Here, we visualize, for the model phage T5, how host recognition and SE can be achieved via the interaction of different phage proteins with the same receptor in the Escherichia coli outer membrane. The receptor for phage T5 was identified as the outer membrane (OM) TonB-dependent transporter (TBDT) FhuA almost 50 y ago. To elucidate the mechanism of SE via potential TBDT structure modulation, we report here the cryo-EM structure of the FhuA–pb5 complex and the X-ray crystal structure of the FhuA–Llp complex. Our structures show that the phage lipoprotein Llp exploits the known allostery in the plug of FhuA in the opposite direction as during ferrichrome import (i.e., from the periplasmic side to the extracellular side).

We succeeded in solving the FhuA–pb5 structure via cryo-EM, using complex purified in decylmaltopyranoside at ∼3.1 Å resolution. The FhuA–Pb5 structure shows that pb5 is an elongated molecule with one end inserted into the extracellular lumen of the FhuA barrel and with its long axis approximately perpendicular to the OM plane. Pb5 inserts four loops (numbered L1 to L4 from the N terminus) into the extracellular lumen of FhuA. With the exception of EL1-EL3, all FhuA loops contact pb5, resulting in a large interface area of ∼2140 Å2 as analyzed via PISA. Pb5 completely fills the extracellular lumen of FhuA and occludes the ferrichrome binding site, explaining why addition of purified pb5 to E. coli inhibits growth under iron-starved conditions. Interestingly, pb5 binding does not cause conformational changes in the TonB box, and the structure of the plug in FhuA–pb5 is identical to that in apo FhuA, despite the fact that ferrichrome and pb5 both contact Phe115 and Tyr116 of the plug. The LPS molecule that is present in FhuA X-ray crystal structures is clearly visible in the cryo-EM map. Interestingly, the region at the other end of pb5 that most likely interacts with pb4 is poorly ordered but present in the cryo-EM density and only visible at low contours. Combined with data placing pb5 at the very tip of the central tail fiber, and the loss of tail tips when detergent-purified FhuA is incubated with T5 (13), we propose that the disorder observed in the pb4-interacting part of pb5 is caused by FhuA binding and leads to the dissociation of the tail tip. To our knowledge, our structural data for FhuA–pb5 provide the most direct evidence to date for the view that DNA transfer does not occur via the FhuA channel, as originally proposed based on single-channel electrophysiology.

> AVEPKEDTITVTAAPAPQESAWGPAATIAARQSATGTKTDTPIQKVPQSISVVTAEEMALHQPKSVKEALSYTPGVSVGTRGASNTYDHLIIRGFAAEGQSQNNYLNGLKLQGNFYNDAVIDPYMLERAEIMRGPVSVLYGKSSPGGLLNMVSKRPTTEPLKEVQFKAGTDSLFQTGFDFSDSLDDDGVYSYRLTGLARSANAQQKGSEEQRYAIAPAFTWRPDDKTNFTFLSYFQNEPETGYYGWLPKEGTVEPLPNGKRLPTDFNEGAKNNTYSRNEKMVGYSFDHEFNDTFTVRQNLRFAENKTSQNSVYGYGVCSDPANAYSKQCAALAPADKGHYLARKYVVDDEKLQNFSVDTQLQSKFATGDIDHTLLTGVDFMRMRNDINAWFGYDDSVPLLNLYNPVNTDFDFNAKDPANSGPYRILNKQKQTGVYVQDQAQWDKVLVTLGGRYDWADQESLNRVAGTTDKRDDKQFTWRGGVNYLFDNGVTPYFSYSESFEPSSQVGKDGNIFAPSKGKQYEVGVKYVPEDRPIVVTGAVYNLTKTNNLMADPEGSFFSVEGGEIRARGVEIEAKAALSASVNVVGSYTYTDAEYTTDTTYKGNTPAQVPKHMASLWADYTFFDGPLSGLTLGTGGRYTGSSYGDPANSFKVGSYTVVDALVRYDLARVGMAGSNVALHVNNLFDREYVASCFNTYGCFWGAERQVVATATFRF;> MSFFAGKLNNKSILSLRRGSGGDTNQHINPDSQTIFHSDMSHVIITETHSTGLRLDQGAGDYYWSEMPSRVTQLHNNDPNRVVLTEIEFSDGSRHMLSGMSMGVGAKAYGIINPQIMSQGGLKTQITASADLSLDVGYFNTGTSGTIPQKLRDGTGCQHMFGAFSGRRGFASSAMYLGGAALYKSAWSGSGYVVADAGTLTIPSDYVRHPGARNFGFNAIYVRGRSCNRVLYGMEGPNYTTGGAVQGASSSGALNFTYNPSNPESPKYSVGFARADPTNYAYWESMGDPNDSANGPIGIYSEHLGIYPSKITWYVTNLVYNGSGYNIDGGLFNGNDIKLSPREFIIKGVNVNNTSWKFINFIEKNFNVGNRADFRDVGCNLSKDSPSTGISGIATFGLPTTESNNAPSIKGGNVGGLHANVVSIYNFLPSASWYVSSNPPKIGNNYGDVWSENLLPLRLLGGSGSTILSGNIVFQGNGSVHVGTVGLDLNSSRNGAIVCTMEFIDDTWLSAGGIGCFNPTEMLSQGAEYGDSRFRIGGNTINKKLHQILSLPAGEYVPFFTIKGTVVNACKLQAAAYNPTPYWVSGLPGSVGQTGYYTLTYYMRNDGNNNISIWLDSSMSNIIGMKACLPNIKLIIQRLTHHHHHH>[2x]MGSHHHHHHGRSMSELIKENMHMKLYMEGTVNNHHFKCTSEGEGKPYEGTQTQRIKVVEGGPLPFAFDILATSFMYGSKT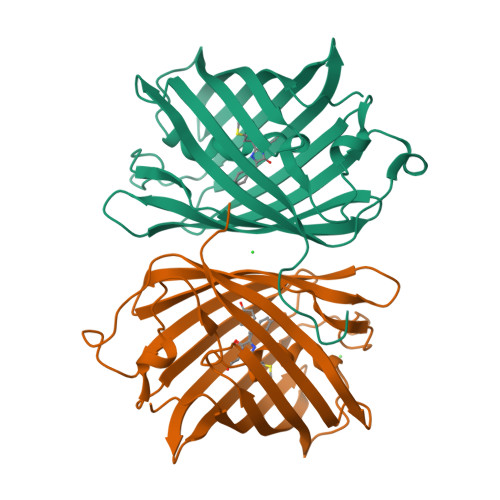FINHTQGIPDFWKQSFPEGFTWERVTTYEDGGVLTATQDTSLQDGCLIYNVKIRGVNFPSNGPVMQKKTLGWEANTEMMYPADGGLEGRNYMALKLVGGGHLICSLKTTYRSKKPAKNLKMPGVYYVDRRLERIKEADKETYVEQHEVAVARYCDLPSKLGHKLN> AMESIGLVEVNSIARGIEAADAMLKAAQVDLLEAKPVCPGKYIVLICGDVAAVQSSVTAGKTMAAHSVLDDFILPNVHPQVLTAISAATPLTLIKALGIIETFSIA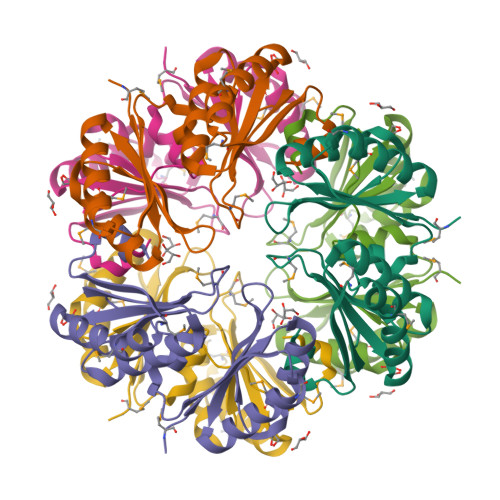SLIVAADTAAKTGQVDLVEIRIGMGIGGKSFVTLTGDVASVESSVAAGVMLASERGMLVDKVVIPSPHDHLKRCLC>GCAGCAGC[8x]

We have analyzed crystal structures of RNA containing CAG repeats in complex with synthetic cyclic mismatch-binding ligands (CMBLs). In total, three X-ray structures consisting of (GCAGCAGC)2-CMBL3a, one structure of (GCAGCAGC)2-CMBL3b and one (GCAGCAGC)2-CMBL4 complex have been analyzed. The models show well-defined interactions between the molecules in which the CMBLs mimic nucleobases as they form pseudo-canonical base pairs with adenosine residues and engage in extensive stacking interactions with neighboring nucleotides. The binding of ligands is associated with major structural changes of the CAG repeats, which is consistent with results of biochemical studies.

The longer linker contains two N-acyl-amino groups and additional constituents: in CMBL3a it is a E-alkene, in CMBL3b it is an Z-alkene, and in CMBL4 it is an aminoalkyl moiety. In more complex cases, in addition to the Watson-Crick pairs, triplex-like interactions are observed between the bulged-out nucleotides (CAG-CMBL3b and CAG-CMBL3a). The 4G and 5C residues can enter the major grove and form additional contacts with the canonical G–C and C–G pairs. In the presence of CMBL3a, the duplex is the most stable, having a melting temperature TM nearly 20°C higher. The X-ray structures show that all three ligands interact with the RNA in very similar manners, but the conformation of the bound CMBL3a is the least distorted from the idealized geometry. The asymmetric trans conformation of the long linker makes the ligand better adjusted to the binding site than the symmetric CMBL3b and CMBL4. This is consistent with the thermal melting observations that CMBL3a forms more stable complexes with the RNA than CMBL3b or CMBL4.> MALTLYQRDDCHLCDQAVEALAQARAGAFFSVFIDDDAALESAYGLR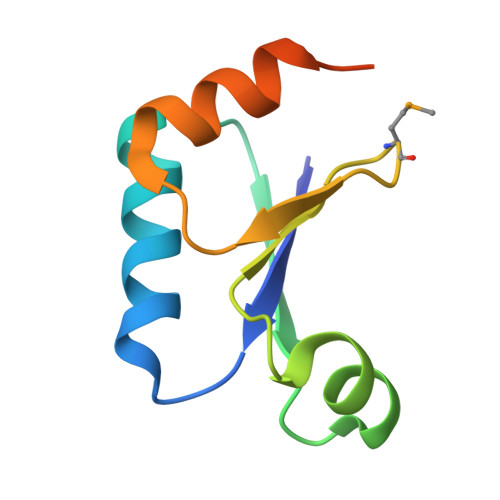VPVLRDPMGRELDWPFDAPRLRAWLDAAPHALEHHHHHHH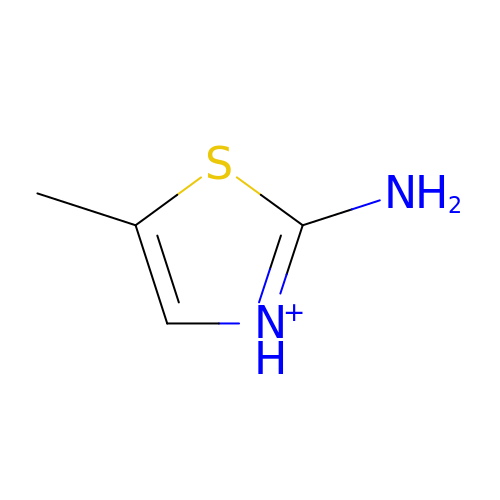2-AMINO-5-METHYLTHIAZOLE | C4 H7 N2 S | GUABFMPMKJGSBQ-UHFFFAOYSA-O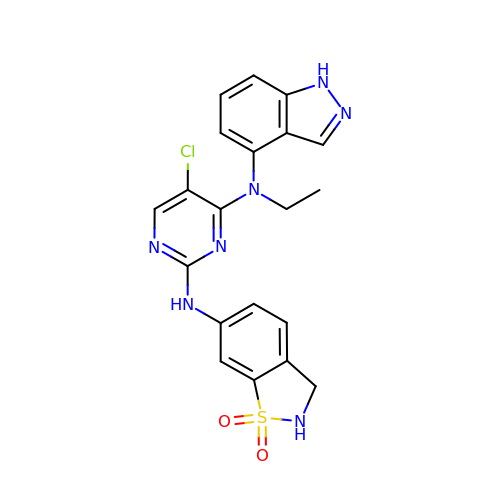5-chloro-N~2~-(1,1-dioxido-2,3-dihydro-1,2-benzothiazol-6-yl)-N~4~-ethyl-N~4~-(1H-indazol-4-yl)pyrimidine-2,4-diamine | C20 H18 Cl N7 O2 S | XZUGISDIVDJNBC-UHFFFAOYSA-N> 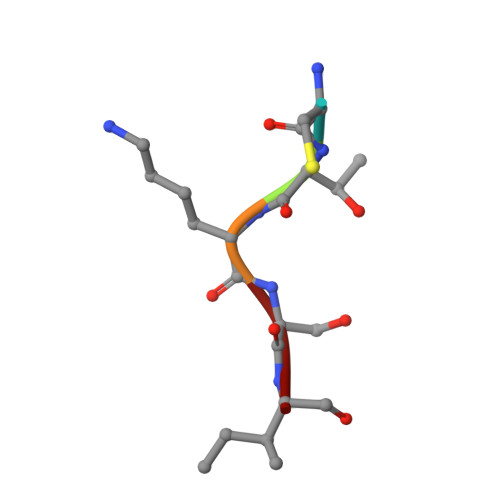CTKSI>MRGSHHHHHHGSARPSNVKPSPHVIMSLEELREATASNRISVIVFTLPDSKRSNEIKEKLRKLAEVFPDVDTYSVDTSTNPEAREWYNITSVPTFVIEKGGEP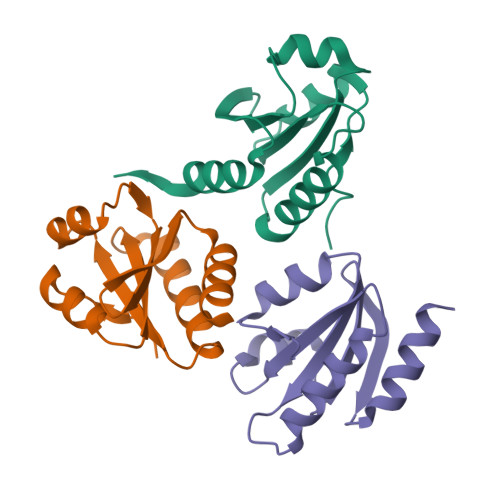LGEVKGPDIDKLRVTLDELLARKLN[3x]> MINVYSNLMSAWPATMAMSPKLNRNMPTFSQIWDYERITPASAAGETLKSIQGAIGEYFERRHFFNEIVTGGQKTLYEMMPPSAAKAFTEAFFQISSLTRDEIITHKFKTVRAFNLFSLEQ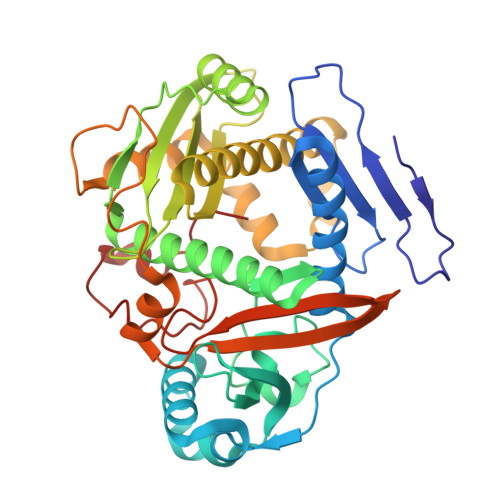QEIPAVIIALDNITAADDLKFYPDRDTCGCSFHGSLNDAIEGSLCEFMERQSLLLYWLQGKANTEISSEIVTGINHIDEILLALRSEGDIRIFDITLPGAPGHAVLTLYGTKNKISRIKYSTGLSYANSLKKALCKSVVELWQSYICLHNFLIGGYTDDDIIDSYQRHFMSCNKYESFTDLCENTVLLSDDVKLTLEENITSDTNLLNYLQQISDNIFVYYARERVSNSLVWYTKIVSPDFFLHMNNSGAININNKIYHTGDGIKVRESKMVPFP> MGPCDIYEAGDTPCVAAHSTTRALYSSFSGALYQLQRGSDDTTTTISPLTAGGIADASAQDTFCANTTCLITIIYDQSGNGNHLTQAPPGGFDGPDTDGYDNLASAIGAPVTLNGQKAYGVFMS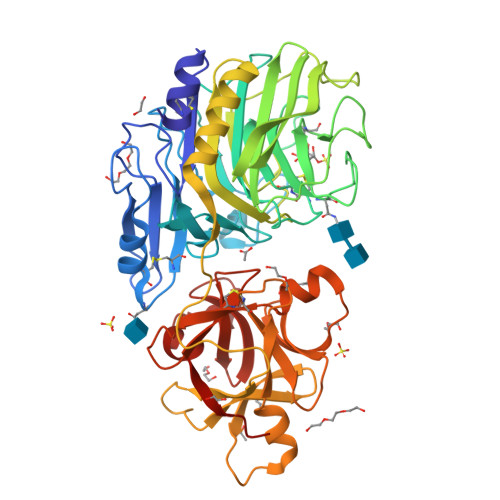PGTGYRNNEATGTATGDEAEGMYAVLDGTHYNDACCFDYGNAETSSTDTGAGHMEAIYLGNSTTWGYGAGDGPWIMVDMENNLFSGADEGYNSGDPSISYRFVTAAVKGGADKWAIRGANAASGSLSTYYSGARPDYSGYNPMSKEGAIILGIGGDNSNGAQGTFYEGVMTSGYPSDDTENSVQENIVAAKYVVGSLVSGPSFTSGEVVSLRVTTPGYTTRYIAHTDTTVNTQVVDDDSSTTLKEEASWTVVTGLANSQCFSFESVDTPGSYIRHYNFELLLNANDGTKQFHEDATFCPQAALNGEGTSLRSWSYPTRYFRHYENVLYAASNGGVQTFDSKTSFNNDVSFEIETAFAS>[3x]PLLNVHIMQGHTPAAKTALLKALSDAVVQSIGAPLASVRAILQEYAAADVIVAGEVGAAMALVNVDLI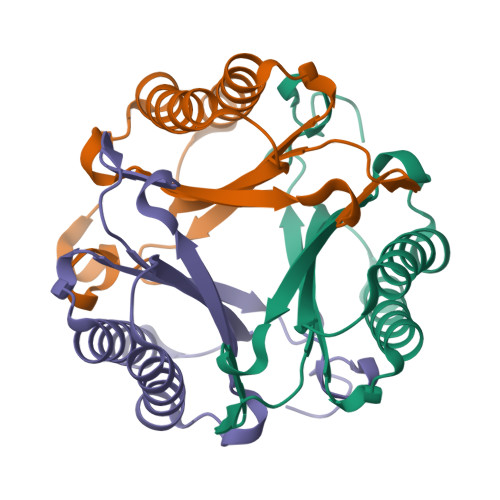AGRTVELKAALILALNQAVSASLGMDGKDVRVVLRDIPKTDMGVANGLSAMAAGR> MIEMKPHPWFFGKIPRAKAEEMLSKQRHDGAFLIR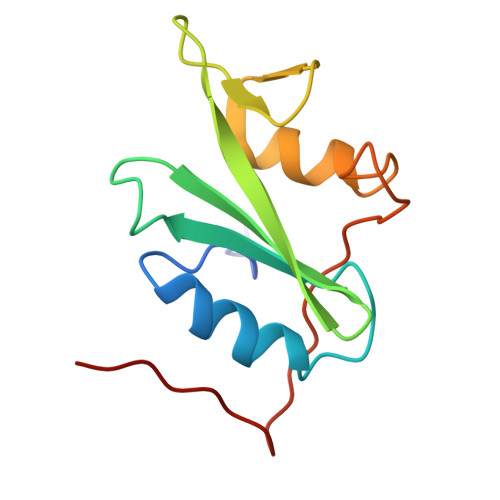ESESAPGDFSLSVKFGNDVQHFKVLRDGAGKYFLWVVKFNSLNELVDYHRSTSVSRNQQIFLRDIEQVPQQPTYVQA> MKQYLELMQKVLDEGTQKNDRTGTGTLSIFGHQMRFNLQDGFPLVTTKRCHLRSIIHELLWFLQGDTNIAYLHENNVTIWDEWADENGDLGPVYGKQWRAWPTPDGRHIDQITTVLNQLKNDPDSRRIIVSAWNVGELDKMALAPSHAFFQFYVADGKLSCQLYQRSCDVFLGLPFNIASYALLVHMMAQQCDLEVGDFVWTGGDTHLYSNHMDQTHLQLSREPRPL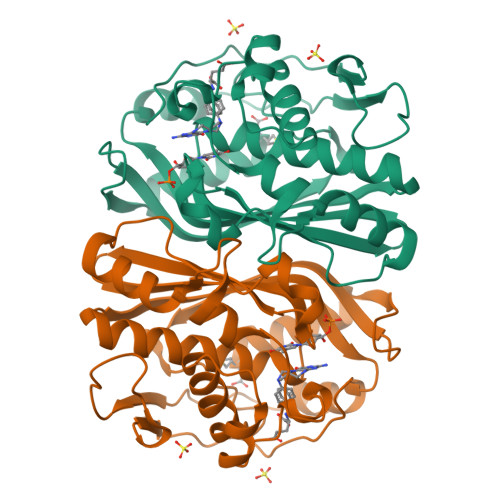PKLIIKRKPESIFDYRFEDFEIEGYDPHPGIKAPVAI>[2x]GPLGSGEPGSARAAVSELMQLFPRGLFEDALPPIVLRSQVYSLVPDRTVADRQLKELQEQGEIRIVQLGFDLDAHGIIFTEDYRTRVLKASDGRPYAGAVQKFLASVLPASGDLSFQQDQMTQTFGFRDSEITHLVNAGVLTVRDAGSWWLAVPGAGRFIKYFVKGRQAVLSMVRKAKYRELLLSELLGRRAPVVVRLGLTYHVHDLIGAQLVDSISTTSGTLLRLPET

Serine/threonine protein kinase 19 (STK19) has been reported to phosphorylate and activate oncogenic NRAS to promote melanomagenesis. STK19 has also been identified as a putative factor involved in the transcription-coupled nucleotide excision repair (TC-NER) pathway. In this study, we determined a 1.32 Å crystal structure of human STK19 protein, revealed that STK19 is a winged-helix (WH) protein instead of a kinase, and performed structural-guided analysis of the STK19 molecular function. STK19 binds more strongly to double-stranded DNA and RNA (dsDNA/dsRNA) than to ssDNA.

We determined the 1.32 Å crystal structure of human STK19, containing residues 31-254. The structure of STK19 reveals a compact fold consisting of three winged helix (WH) domains (WH1-WH3) packed together. Notably, the WH3 nucleic acid recognition helix (WH3-H3) is less accessible compared to WH1-H3 and WH2-H3, owing to its proximity to WH1-H2. The STK19 protein in solution is monomeric, as suggested by analytical gel filtration, run in parallel with dimeric Glutathione S-transferase (GST) protein of similar size and with gel filtration standards. This conclusion is also supported by chemical crosslinking using Disuccinimidyl Suberate (DSS). Electrostatic surface analysis of the STK19 structure reveals a large patch of basic residues centered on the WH3-H1 helix. These residues include R183, K186, K190, R192, R200, and K201 of the helix WH3-H1, K203 and R205 in the following loop, and R215, R216, and R222 in the H2-H3 loop of the WH3 domain. Mutations of these conserved residues, namely K186E, R200E/K201E/K203E, and R215E/R216E, abolished dsDNA binding. We selected and purified to homogeneity four STK19 protein variants harboring the patient mutation. Of the investigated mutations, K186N, R200W, and R215W significantly compromised STK19 dsDNA binding ability.>[5x]GMSHIQRETSCSRPRLNSNLDADLYGYRWARDNVGQSGATIYRLYGKPNAPELFLKHGKGSVANDVTDEMVRLNWLTAFMPLPTIKHFIRTPDDAWLLTTAIPGKTAFQVLEEYPDSGENIVDALAVFLRRLHSIPVCNCPFNSDRVFRLAQAQSRMNNGLVDASDFDDERNGWPVEQVWKEMHKLLPFSPDSVVTHGDFS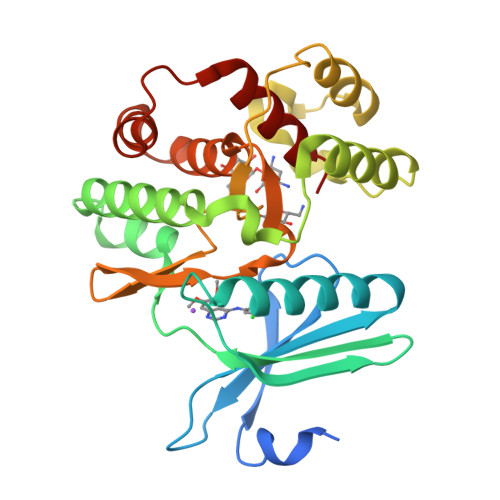LDNLIFDEGKLIGCIDVGRVGIADRYQDLAILWNCLGEFSPSLQKRLFQKYGIDNPDMNKLQFHLMLDEFF>GPLGSTSDILHRMVIHVFSLQQMTAHKIYIHSYNTATIFHELVYKQTKIISSNQELIYEGRRLVLEPGRLAQHFPKTTEENP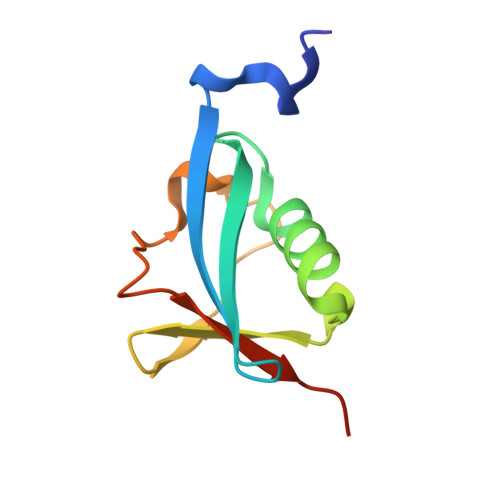IFVVSLERPHRD[2x]> LDL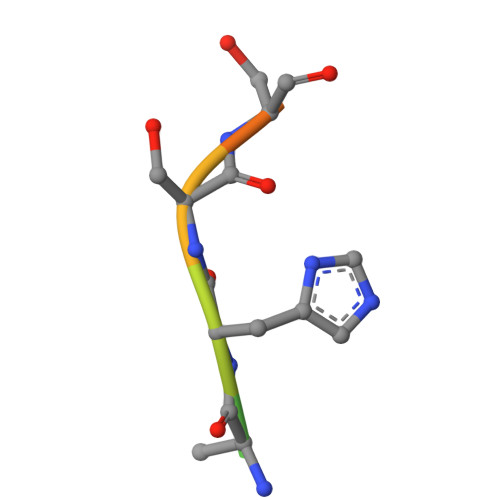AHSSESQ>GHMSPNYDKWEMERTDITMKHKLGGGQYGEVYEGVWKKYSLTVAVKTLKEDTMEVEEFLKEAAVMKEIKHPNLVQLLGVCTREPPFYIITEFMTYGNLLDYLRECNRQEVNAVVLLYMATQISSAMEYLEKKNFIHRDLAARNCLVGENHLVKVADFGLSRLMTGDTYTAPAGAKFPIKWTAPESLAYNKFSIKSDVWAFGVLLWEIATYGMSPYPGIDLSQVYELLEKDYRMERPEGCPEKVYELMRACWQWNPSDRPSFAEIHQAFETMFQESSISDEVEKELGK[2x];> EAIFAAPFAKK

BCR–Abl is a constitutively activated form of the nonreceptor tyrosine kinase c-Abl. The improper activation of the Abl tyrosine kinase results in chronic myeloid leukemia (CML). The recognition of an inactive conformation of Abl, in which a catalytically important Asp-Phe-Gly (DFG) motif is flipped by approximately 180° with respect to the active conformation, underlies the specificity of the cancer drug imatinib, which is used to treat CML. Our results suggest that interconversion between distinctly different inactive conformations is a characteristic feature of the Abl kinase domain.

The other crystal form of the H396P mutant has two molecules in the asymmetric unit that are in different conformations. The first of these molecules (molecule D) is in an inactive conformation with a flipped DFG motif (DFG-Asp Out/αC-Glu In) despite the presence of the ATP analog in the nucleotide-binding site. Previously, DFG-Asp Out conformations of Abl have only been seen in the presence of high-affinity kinase inhibitors such as imatinib and PD166326. The appearance of the DFG-Asp Out conformation in the presence of a nucleotide analog shows that this conformation is an accessible state of the kinase domain of Abl and is not induced only by the binding of high-affinity kinase inhibitors. The second molecule (molecule E) in this crystal form is in an intermediate conformation, with helix αC partially swung out of the active site and with disruption of the conserved ion pair between Glu 286 and Lys 271 (DFG-Asp Out/αC-Glu Out). Molecules E and G were obtained from the same crystal form of Abl and are very similar, except for the presence of either the ATP-peptide analog (molecule E) or the kinase inhibitor PD166326 (molecule G). In these structures, the kinase adopts a conformation intermediate between αC-Glu In and αC-Glu Out: while helix αC is not rotated out of the active site of the kinase, a rotation of the side chain of Glu 286 has occurred, resulting in the breakage of the Glu 286–Lys 271 salt bridge. The conformation of Abl represented by molecules E and G suggests a mechanism by which Abl can interconvert between αC-Glu In and αC-Glu Out conformations.>[2x]AQHPDSVIYQTSLMSALLSGVYEGETTIADLLAHGDFGLGTFNEL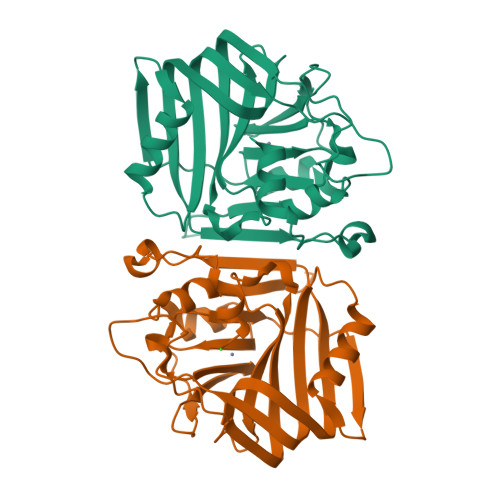DGEMIAFSSQVYQLRADGSARAAKPEQKTPFAVMTWFQPQYRKTFDTPVSRQQIHDVIDQQIPSDNLFCALRIDGNFRHAHTRTVPRQTPPYRAMTDVLDDQPVFRFNQREGVLVGFRTPQHMQGINVAGYHEHFITDDRQGGGHLLDYQLESGVLTFGEIHKLMIDLPADSAFLQANLHPSNLDAAIRSVEN We also present structures of AvaR1, in isolation (2.4 Å resolution), in complex with avenolide (2.0 Å resolution), and bound to a synthetic DNA oligonucleotide (3.09 Å resolution) derived from its natural binding site. The overall structure is reminiscent of that of other TetR-family transcriptional repressors, and consists of an obligate homodimer. Each monomer is entirely helical and consists of a DNA-binding domain (DBD; composed of α helices 1–4), and a ligand-binding domain (LBD; consisting of α helices 5–13). The dimer interface is formed via interactions between the two LBDs and is formed mainly through hydrophobic packing interactions.

Co-crystallization efforts for AvaR1 bound to avenolide yielded crystals that diffracted to 2.0 Å resolution, and crystallographic phases were determined using molecular replacement (Thorn and Sheldrick, 2013). Clear density for the entire hormone can be visualized bound to the LBD of both monomers in the homodimer. Notably, the structure of AvaR1 undergoes conformational shifting upon ligand binding, and a structure-based superposition against the ligand-free structure illustrates that binding of the hormone results in an ~10o shift in the DBD of each monomer. This shift results in an increase in the distance between the two DBD in the dimer upon binding of the ligand, which would preclude DNA binding by the ligand-bound homodimer. Additional local changes between the two structures included the movement of Gln165, which swings into the binding pocket to make hydrogen-bonding interactions with the lactone ring, as well with Gln64. Last, Thr108, which is harbored on helix α6, also moves to accommodate interactions with the hormone. The indole side chain of Trp127 likewise shifts to increase the volume of the binding cavity. Other interactions include hydrogen bonds between Thr131 and the C10 hydroxy, and an interaction between Thr162 and the lactone ring of avenolide. The superimposition suggests that the new contacts formed by these residues are likely to couple hormone binding to the conformational shift between the two monomers of AvaR1. Specifically, movement of Gln64 and Thr108 into the ligand-binding cavity of AvaR1 upon engagement of the hormone results in the displacement of helix α6 away from the pocket.

>GSENLYFQSGAVARQERAIRTRQTILVAAAEVFDEVGYEAATISDVLKRSGVTKGALYFHFTSKQELAQAVLAEQVASLPRVPEQELKLQQSLDEALLLAHLLREGTGDPIVQGSVRLTVDQGSPRDHLNRRVPMQAWTEHTQSLFEEARAKGEILPHADVEALAKLFVGAFTGVQVLSRIMTGRADLAERVADLYRHLMPSFAMPGILVRLDFSPERGSRVYEAAMKQRESAAASTTDAARTLE[8x]Sterile alpha motif and HD-domain containing protein 1 (SAMHD1) is a dNTP triphosphohydrolase that catalyses the breakdown of dNTPs to constituent 2′-deoxynucleoside and triphosphate, and is therefore an important regulator of cellular nucleotide homeostasis in mammalian cells. SAMHD1 dNTP triphosphohydrolase catalytic activity requires assembly into homo-tetramers. Sequences at the N- and C-termini of the HD domain stabilise inter-monomer protein-protein interactions and incorporate four pairs of allosteric, AL1 and AL2, nucleotide-binding sites. Nucleotide binding at these sites promote tetramer-assembly and regulate SAMHD1 through combined binding of G-based (AL1) and 2’-deoxynucleoside (AL2) triphosphates.

First, that dNTP hydrolysis occurs within the confines of the D2 symmetrical State-I tetramer where each Dimer-2 pair is in the tense state, substrates are bound at the Fe-Mg bimetallic centre and the phosphate, sugar and base-binding active site residues are engaged with the dNTP. This configuration is observed in both the crystal and our cEM structures of SAMHD1-inhbitor complexes that have the State-I conformation with the attacking nucleophile hydroxyl positioned on the substrate Pα and likely represent the catalytic state prior to adduction and formation of a transition state.

>[4x]MQRADSEQPSKRPRCDDSPRTPSNTPSAEADWSPGLELHPDYKTWGPEQVCSFLRRGGFEEPVLLKNIRENEITGALLPCLDESRFENLGVSSLGERKKLLSYIQRLVQIHVDTMKVINDPIHGHIELHPLLVRIIDTPQFQRLRYIKQLGGGYYVFPGASHNRFEHSLGVGYLAGCLVHALGEKQPELQISERDVLCVQIAGLCHDLGHGPFSHMFDGRFIPLARPEVKWTHEQGSVMMFEHLINSNGIKPVMEQYGLIPEEDICFIKEQIVGPLESPVEDSLWPYKGRPENKSFLYEIVSNKRNGIDVDKWDYFARDCHHLGIQNNFDYKRFIKFARVCEVDNELRICARDKEVGNLYDMFHTRNSLHRRAYQHKVGNIIDTMITDAFLKADDYIEITGAGGKKYRISTAIDDMEAYTKLTDNIFLEILYSTDPKLKDAREILKQIEYRNLFKYVGETQPTGQIKIKREDYESLPKEVASAKPKVLLDVKLKAEDFIVDVINMDYGMQEKNPIDHVSFYCKTAPNRAIRITKNQVSQLLPEKFAEQLIRVYCKKVDRKSLYAARQYFVQWCADRNFTKPQDGDVIAPLITPQKKEWNDSTSVQNPTRLREASKSRVQLFKDDPM In the present study, we describe a new artificial binding protein scaffold that we have named Adhiron. This scaffold is based on a consensus sequence of plant-derived phytocystatins, which are small (ca. 100 aa) protein inhibitors of cysteine proteases. The overall structure comprises the characteristic cystatin family fold of a four-strand anti-parallel β-sheet core with a central helix.

The Adhiron scaffold was derived from the phytocystatin consensus protein by initial N-terminal truncation to a 92 amino acid sequence which we refer to as the full-length Adhiron scaffold, or Adhiron92. We have determined the crystal structure of the full-length Adhiron92 scaffold by X-ray crystallography. Amino acids 1–10 and 90–92 are not visible in the electron density maps presumably as they are disordered. The Adhiron structure is compact with limited unstructured loops and this is consistent with the very high melting temperature of this consensus protein. The thermal stability of the Adhiron92 and Adhiron81 scaffolds was tested by DSC and both gave identical profiles with a melting temperature of 101°C.

> ENSLEIEELARFAVDEHNKKENALLEFVRVVKAKEQVVAGTMYYLTLEAKDGGKKKLYEAKVWVKPWENFKELQEFKPV6-{[(3S,4S)-4-{2-[(2-fluorobenzyl)amino]ethoxy}pyrrolidin-3-yl]methyl}-4-methylpyridin-2-amine 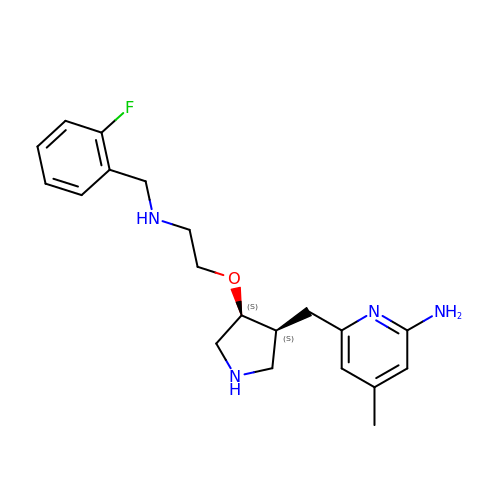| C20 H27 F N4 O | PMZVISPCVPVOFN-QFBILLFUSA-N> GPEATLGSGNLRMAVMLPEGEDLNEWVAVNTVDFFNQINMLYGTITDFCTEESCPVMSAGPKYEYHWADGTNIKKPIKCSAPKYIDYLMTWVQDQLDDETLFPSKIGVPFPKNFMSVAKTILKRLFRVYAHIYHQHFDPVIQLQEEAHLNTSFKHFIFFVQEFNLIDRRELAPLQELIEKLTSKDR;> GPKDEERRESRIQSYSPQAFKFFMEQHVENV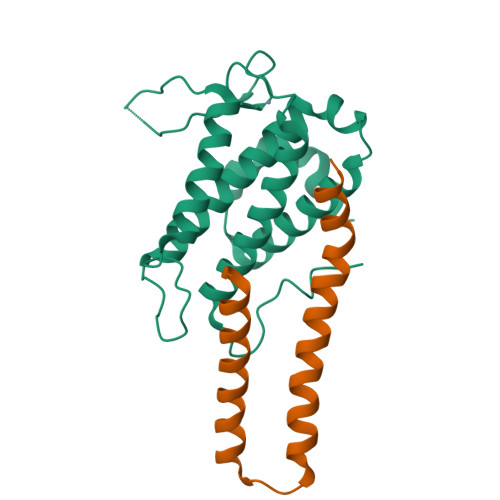LKSHQQRLHRKKQLENEMMRVGLSQDAQDQMRKMLCQKESNYIRLKRAKMDKSM> HMHKRPKRP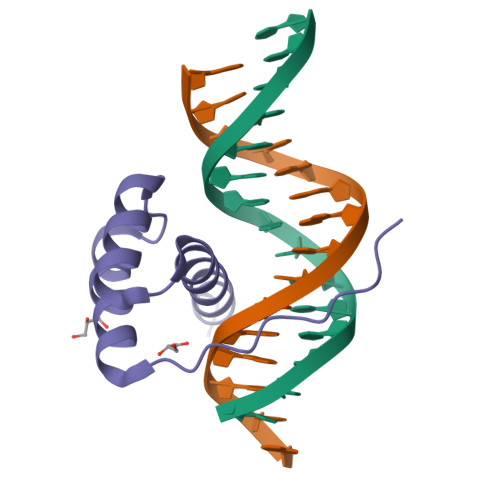RTILTTQQRRAFKASFEVSSKPCRKVRETLAAETGLSVRVVQVWFQNQRAKMKKLARR>MNWTVDIPIDQLPSLPPLPTDLRTRLDAALAKPAAQQPTWPADQALAMRTVLESVPPVTVPSE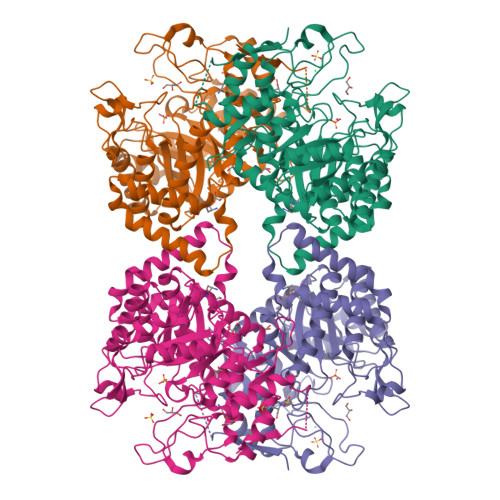IVRLQEQLAQVAKGEAFLLQGGDCAETFMDNTEPHIRGNVRALLQMAVVLTYGASMPVVKVARIAGQYAKPRSADIDALGLRSYRGDMINGFAPDAAAREHDPSRLVRAYANASAAMNLVRALTSSGLASLHLVHDWNREFVRTSPAGARYEALATEIDRGLRFMSACGVADRNLQTAEIYASHEALVLDYERAMLRLSDGDDGEPQLFDLSAHTVWIGERTRQIDGAHIAFAQVIANPVGVKLGPNMTPELAVEYVERLDPHNKPGRLTLVSRMGNHKVRDLLPPIVEKVQATGHQVIWQCDPMHGNTHESSTGFKTRHFDRIVDEVQGFFEVHRALGTHPGGIHVEITGENVTECLGGAQDISETDLAGRYETACDPRLNTQQSLELAFLVAEMLRD[2x]>METYIKLDKLGEGTYATVYKGKSKLTDNLVALKEIRLEHEEGAPCTAIREVSLLKDLKHANIVTLHDIIHTEKSLTLVFEYLDKDLKQYLDDCGNIINMHNVKLFLFQLLRGLAYCHRQKVLHRDLKPQNLLINERGELKLADFGLARAKSIPTKTYDNEVVTLWYRPPDILLGSTDYSTQIDMWGVGCIFYEMATGRPLFPGSTVEEQLHFIFRILGTPTEETWPGILSNEEFKTYNYPKYRAEALLSHAPRLDSDGADLLTKLLQFEGRN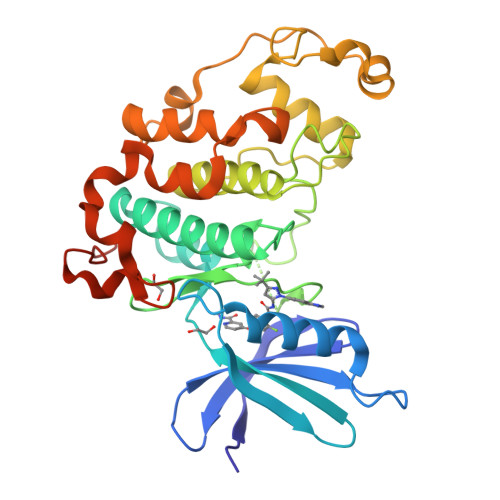RISAEDAMKHPFFLSLGERIHKLPDTTSIFALKEIQLQKEASLRSAHHHHHH[2x]> GPTIEE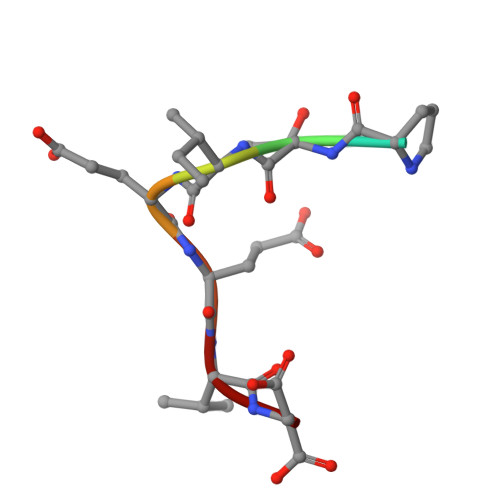VD>DAAQPARRANGSEWSYTNILTGPETWHEHYKNMCSGYYQSPIDLKTDISTLDLKLKTVIIYRNTSSTETTTIQNNGHSAEVKFPRNTWFISFDGILDYKYEIIQMHFHWGNTDDRGSEHTIDGFRFPLEGHIVSFRRQMYSSPSEAIGRPGGLAVLGIMHQIVE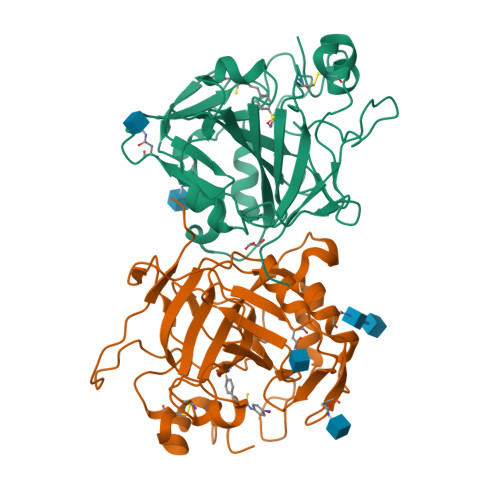SIKYEQTAFKAYNNFSGVLNSQFVPPNNSTIDDINLALLLSLLNPSRYFRYLGSLTTPPCTENVLWTVFIDPVLITREQINLFRNLPYGSNEKQTRMGDNFRPIQLLNPIDTLASRTLYRATARGGPEQKLISEEDLNSAVDHHHHHH[2x]> SICSEPKKVGRCL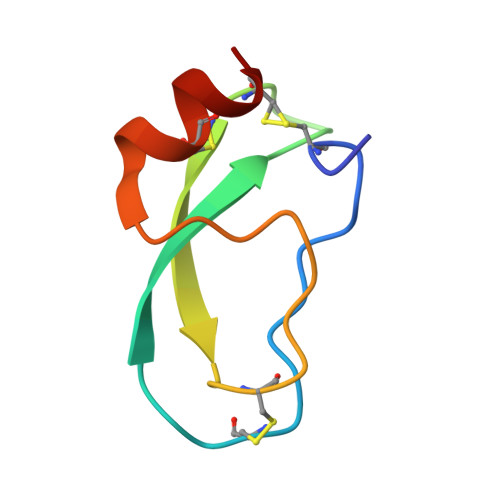GYFPRFYFDSETGKCTPFIYGGCGGNGNNFETLHQCRAICRA> GHMPEYDYLFKLLLIGDSGVGKSCLLLRFADDTYTESYISTIGVDFKIRTIELDGKTIKLQIWDTAGQERFRTITSSYYRGAHGIIVVYDVTDQESYANVKQWLQE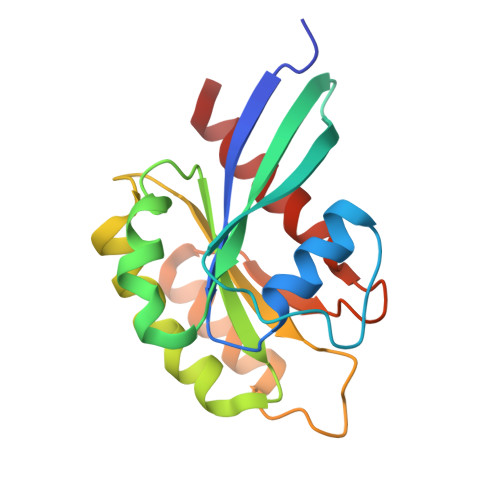IDRYASENVNKLLVGNKSDLTTKKVVDNTTAKEFADSLGIPFLETSAKNATNVEQAFMTMAAEIKKRMG> MKRALGFLSLLVIFASLLVALSPEYGIKFGVGGEDWLKYRYTDNYYIEHGIEEVGGTNIVTDIVFDYRGYDTLGEATVLFTAIAGAVALLRP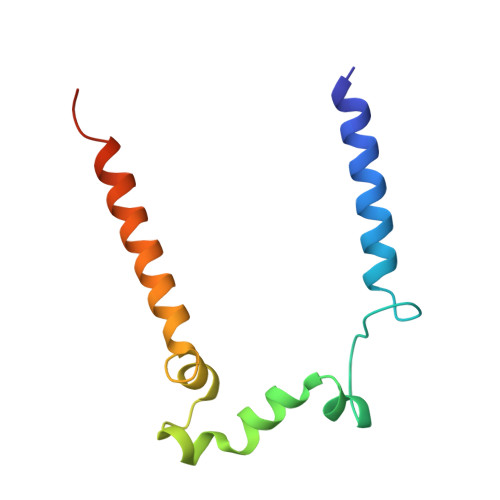WRREENE>[10x]DYKDDDDKLDRADILYNIRQTSRPDVIPTQRDRPVAVSVSLKFINILEVNEITNEVDVVFWQQTTWSDRTLAWNSSHSPDQVSVPISSLWVPDL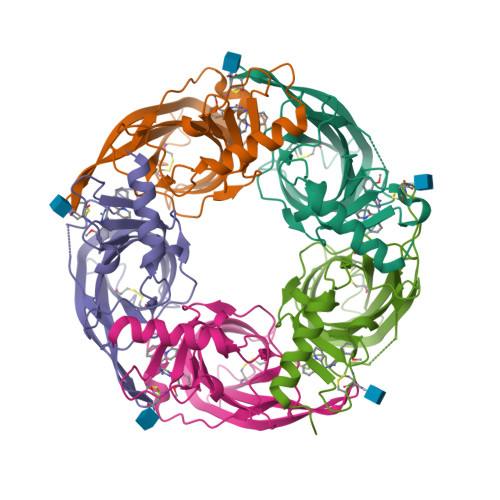AAYNAISKPEVLTPQLARVVSDGEVLYMPSIRQRFSCDVSGVDTESGATCRIKIGSWTHHSREISVDPTTENSDDSEYFSQYSRFEILDVTQKKNSVTYSCCPEAYEDVEVSLNFRKKGRSEIL>MAQRRPAGKKVPFQKDSFLKQFEKLSQSRKQHVLLESARGGRYSIAGLDPIATVKGKDGITTIKHGDEMLFKEGDPLRAFHSWFKTLETETDHELPDFQGGAIGFLSYDYARYIENFKMLSLDDLETPDIYFLVFDDIAVYDHQEESLWLITHVNGTDNSADVKLSELERMWLTELPAVPSREMKRETDGSFAAPFTEDGFSQAVEKIKQYIASGDVFQVNLSIRQSQSLSVHPYQIYKTLREVNPSPYMAYLETPDFQIICGSPELLVSKKGKLLETRPIAGTRSRGKTDEEDESLANELIHNEKERAEHVMLVDLERNDLGRVSRYGSVRVNEFMAIEKYSHVMHIVSNVQGELQDGYDAVDIIHAVFPGGTITGAPKVRTMEIIEELEPTRRGLYTGSIGWFGYNHDLQFNIVIRTIYATGGQAFMQSGAGVVIDSVPKHEYRESFKKAFAMQKALE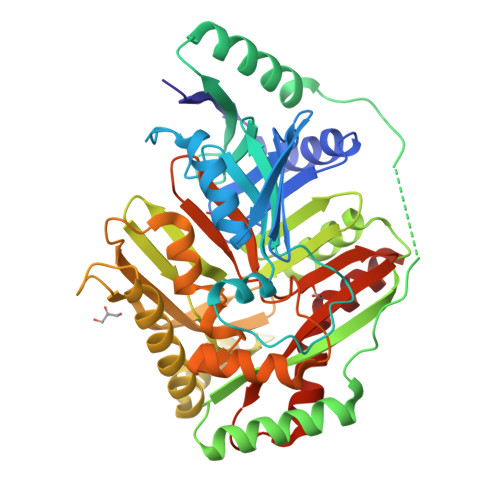LSEEETKIR[3x]> GSVHKHTGRNCGRKFKIGEPLYRCHECGCDDTCVLCIHCF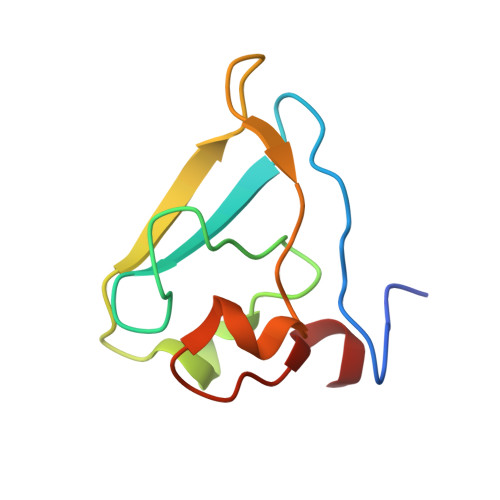NPKDHVNHHVCTDICTEFTSGICDCGDEEAWNSPLHCKAEEQ> GAACGACACTGACGGAGACTC;> CCGTCA;> TCGAGTCT;> GTGTCGT

In this work, we exhaustively probe the ability of all 36 immobile HJ sequences to form DNA crystals in two different designed systems. Three separate self-assembling DNA crystal systems are described in this report: the “4 × 5” and “4 × 6” designs (collectively referred to as the 4 × N systems), and a third construct with a “scrambled” sequence variant of the 4 × 6 lattices. Self-assembly was mediated by three constituent oligonucleotides: (S1) containing four sequence repeats of either 5 or 6 bases; (S2) composed of 21 bases containing complementary regions to both (S1); and (S3) which forms the second junction crossover. The HJ serves as the fundamental component at the core of each unit, and the ultimate assembly of the full lattice is facilitated by the complementary 2-base sticky ends that tail each duplex.

Because the 4 × 6 system yielded R3 symmetry in 5 of 17 junctions, we considered whether the downstream sequences adjacent to the junction could play a role in crystallization efficiency, junction angle, and symmetry preference, or if the HJ alone was the singular determinant. To investigate this possibility, we designed “scrambled” sequences with targeted base substitutions, while maintaining GC content, along each “stem”. Contrary to the buffer preference observed with the native P32 crystals, the scrambled systems exhibited an exclusive preference towards low salt buffers, much like the native R3 crystals. Remarkably, only J1 and J2 retained the P32 symmetry, with all others yielding an R3 lattice. It is also noteworthy that J1 and J2 (P32), along with the R3 systems, also shared a preference for low salt conditions, unlike the original P32 crystals. There appeared to be only a marginal difference in the average cell lengths in the R3 scramble crystals (a = b = 113.04 c = 51.10) relative to the native 4 × 6 sequences: the a, b axis trended ~2 Å shorter and c ~1.3 Å longer, whereas in the J1 and J2 cases, the crystals were in good agreement with the original 4 × 6 motif. By contrast, the calculated angle for the P32 crystals was 58.05° (n = 2, σ = 1.39), compared with 54.60° (n = 16, σ = 1.44), a less accurate average due to a small sample size, so we posit that 54.60° more closely reflects the average observed angles in the 4 × 6 systems. However, in the majority of the crystal structures reported here, the cacodylate anion indeed fits best into the electron density map of our X-ray structures, due to the presence of sodium cacodylate in the crystallization solution.The genome is replicated via a negative-sense RNA intermediate by 3Dpol, the viral RNA-dependent RNA polymerase (RdRP). For this, 3Dpol uses the viral protein 3B, in this context usually termed VPg (viral protein genome-linked), as a primer. Crystal structures have been reported of 3Dpol of the enteroviruses CVB3, PV, EV71, HRV1B, HRV14, and HRV16, and of the aphthovirus FMDV. These enzymes adopt a classical right hand architecture, with fingers, palm and thumb subdomains providing the correct geometrical arrangement of substrate molecules and metal ions at the polymerase active site for catalysis. Given its critical role in genome replication, 3Dpol is regarded as an attractive target for antiviral drugs.

Co-crystals of EMCV 3Dpol with the inhibitor were not obtained, but the structure of the complex of CVB3 3Dpol with GPC-N114 was obtained by X-ray crystallography at 2.9 Å resolution. The analysis of the difference electron density maps revealed the presence of extra densities to position the inhibitor within a pocket located at the bottom of the template channel, mimicking the position of the template acceptor nucleotide, the nucleotide which will base-pair with the incoming nucleotide. The compound bound in a conformation that perfectly fitted the shape of the pocket formed by residues L107, E108, L110, D111, T114 of motif G, R188, Y195, H199 of motif F, T294, S295, I296 of motif B and Y327 of motif A. Among all contacts observed, the stacking interaction between Y195 and the central chlorophenyl ring of GPC-N114 appeared to be an important determinant of binding. This tyrosine is strictly conserved in enterovirus polymerases but not conserved in FMDV and EMCV. The first 2-cyano-4-nitrophenyl ring was oriented towards the entrance of the template channel, interacting with residues of motif G and B of CVB3 3Dpol, whereas the second 2-cyano-4-nitrophenyl ring appeared partially exposed to the solvent, occupying the position expected for the template acceptor base. Structural comparisons between unbound and GPC-N114-bound CVB3 3Dpol revealed that the polymerase did not undergo any major conformational change upon binding of the compound. This preservation of the template cavity conformation extended to the interacting side chains, which maintained their native conformation upon GPC-N114 binding. GPC-N114 did not compete with incoming NTPs, but interfered with productive binding of the template-primer to 3Dpol in a primer elongation assay. This is in agreement with the crystallographic studies of the CVB3 3Dpol–GPC-N114 complex which revealed that the binding site of the compound is located at the junction of the palm and the fingers domains, and overlaps partially with the binding site of the template. Hence, GPC-N114 is the first reported picornavirus polymerase inhibitor that binds the site of the template acceptor nucleotide.

> GEIEFIESSKDAGFPVINTPSKTKLEPSVFHQVFEGNKEPAVLRSGDPRLKANFEEAIFSKYIGNVNTHVDEYMLEAVDHYAGQLATLDISTEPMKLEDAVYGTEGLEALDLTTSAGYPYVALGIKKRDILSKKTKDLTKLKECMDKYGLNLPMVTYVKDELRSIEKVAKGKSRLIEASSLNDSVAMRQTFGNLYKTFHLNPGVVTGSAVGCDPDLFWSKIPVMLDGHLIAFDYSGYDASLSPVWFACLKMLLEKLGYTHKETNYIDYLCNSHHLYRDKHYFVRGGMPSGCSGTSIFNSMINNIIIRTLMLKVYKGIDLDQFRMIAYGDDVIASYPWPIDASLLAEAGKGYGLIMTPADKGECFNEVTWTNATFLKRYFRADEQYPFLVHPVMPMKDIHESIRWTKDPKNTQDHVRSLCLLAWHNGEHEYEEFIRKIRSVPVGRCLTLPAFSTLRRKWLDSFHHHH>MHHHHHHHMAVKKSVGDLHKADLEGKRVFVRADLNVPLDKATLAITDDTRIRAAVPTLKYLLDNGAKVLLTSHLGRPKGGPEDKYRLTPVVARLSELLGKPVTKVDDCIGPEVEKAVGAMKNGELLLLENVRFYKEEEKNEPEFAKKLAANADLYVNDAF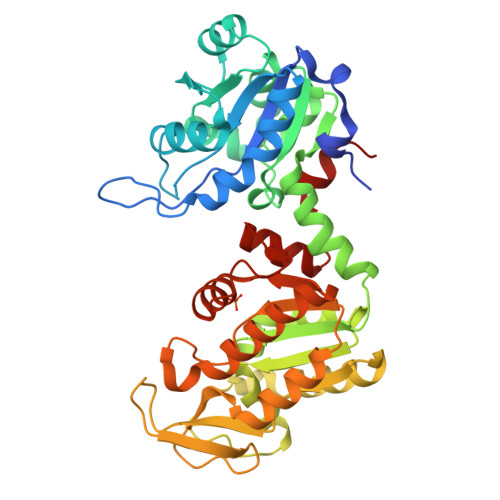GTAHRAHASTEGVTKFLKPSVAGFLLQKELDYLDGAVSNPKRPFVAIVGGSKVSSKITVIEALMEKCDKIIIGGGMIFTFYKARGLKVGSSLVEDDKIELAKKLEEMAKAKGVQLLLPTDVVVADKFDANANTQTVPITAIPDGWMGLDIGPDSVKTFNDALADAKTVVWNGPMGVFEFPKFANGTVSIANTLAGLTPKGCITIIGGGDSVAAVEQAGVAEKMSHISTGGGASLELLEGKVLPGVAALDEK[2x]> GGIGRHTPYGNQTDYRIFELNKRLQNWTEECDNLWWDAFTTEFFEDDAMLTITFCLEDGPKRYTIGRTLIPRYFRSIFEGGATELYYVLKHPKEAFHSNFVSLDCDQGSMVTQHGKPMFTQVCVEGRLYLEFMFDDMMRIKTWHFSIRQHRELIPRSILAMHAQDPQMLDQLSKNITRCGLSNSTLNYLRLCVILEPMQ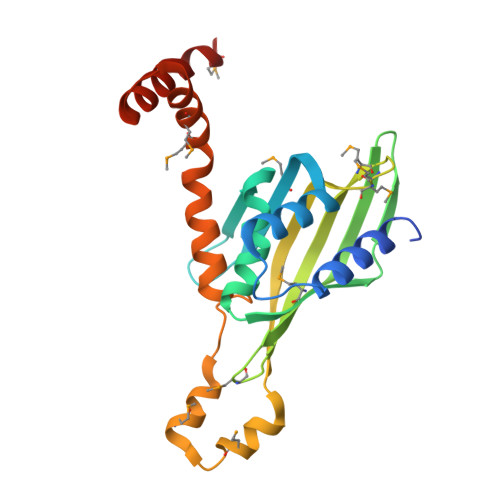ELMSRHKTYSLSPRDCLKTCLFQKWQRMVAPP>[2x]MARTLFLEEGPMFFEKIAPYTYRIPRQGKMRVDAVFFASKEILKDLEAENYASLQQLMNVATLPGIVEPALAMPDIHWGYGFPIGGVAAFDPEEGGVVSPGGVGFDINCGVRLLASHLTLEDLLPRQKELADALYRLVPSGVGSERRDVRFSKRELKEILKEGAGWLVKRGYGYPEDVRFIESQGRLPWANPDK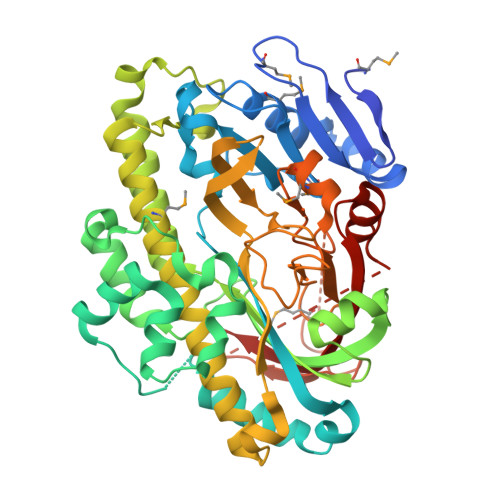VSERAFERGAPQIGTLGSGNHFLEVQYVDEVYDEEAALAFGLFKGQVTVLIHTGSRGLGHQVCQDYVERFLKVAPRYGIELVDKQLAAAPIKSPEGQDYLQAMAAAANFAFANRQLIAHFVREAFEKVGFTPRDHGLRVLYDLAHNNAKFEEHRGRRVLVHRKGATRAFGPGHPEVPEEYRRVGQPVLVPGDMGRYSYVLAGTEKAMEVSFGSSCHGAGRKMSRHQAKKVARERNLVKELAERGILVRAATRATVDEEMPEAYKDVSLVVEAVEGAGIGKKVARLRPLIVVKG> GLVPRGSHMYAELSPGTKKVYTQVRYLDDYHWEIEGSTIT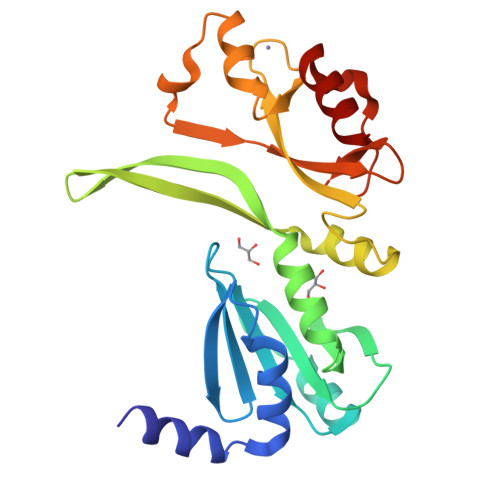GIHKKSNVKVVIDVAKNREEADSLAGKDVNGIHIVAIPDNGVFYIKNGSFVLTYRYLKATLADINDHIVWSGFKVVEDNGKLVQEDVYEYLGAALVNHIKNNALAGQDYIFWQFYKCEECGKYVDIENLEAHLREHGIKLHEKSEEHYEVFELNFREGKVFDKFGGEVPMDKFSSEAREFIKEVLS>[4x]MARIIENNVGGVALTFDDVLLRPEFSNVLPRDIDISTRIAKDFTLNLPIMSAAMDQVTDSRLAIAMAQAGGLGVIHRNFSPSEQVAQVHQVKKFESGGVKDIERSQLNPNATKDSKGRLRVAAAVSVAKDIADRVGPLFDVNVDLVVVDTAHGHSQKVLDAVVQIKKNFPSLLVMAGNIATAEGALALIDAGADIIKVGIGPGSICTTRVVTGVGCPQLSAIMSVVEVAERAGVAIVADGGIRFSGDIAKAIAAGSACVMIGSLLAGTDESPGDIFLYQGRSFKSYRGMGSVAAMERGSSARYSQDGVTDVLKLVPEGIEGRVPYKGPIASVLHQMSGGLKSSMGYVGASNIEEFQKKANFIRVSVAGLRESHVHDVKITRESPNYSETI

Inosine 5′-monophosphate dehydrogenase (IMPDH) is the first and rate-limiting step in guanine nucleotide biosynthesis, controlling the gateway to guanine nucleotides. IMPDH catalyzes the oxidation of inosine 5′-monophosphate to xanthosine 5′-monophosphate (XMP) with a concomitant reduction of NAD+ to NADH. A monomer consists of two domains, namely, the catalytic domain, which is an eight-fold β/α barrel, and a subdomain, including two tandem cystathione-synthetase motifs (CBS domain or Bateman domain), which protrudes from the corners of the homotetramer. IMPDH is also a promising target for antibacterial drug discovery.

In this study, a CLas IMPDH variant without the CBS domain (CLas IMPDHΔ98-201) was designed. To get the CBS deletion construct, 104 residues (98-201aa) were replaced with a G amino acid, and the catalytic residue Cys309 was completely conserved. The crystal structure of CLas IMPDHΔ98-201 was determined in the apo form. Crystals of CLas IMPDHΔ98-201 appeared after 3 days at 293 K. The resolution of the diffracting crystal was 2.55 Å. Finally, the structure was refined to 2.55 Å resolution by using the PHENIX software. This crystal protein existed as a homotetramer, which is well conserved in other IMPDHs. The space group of CLas IMPDHΔ98-201 was C121, and the unit-cell parameters for CLas IMPDHΔ98-201 were a = 143.13, b = 134.86, and c = 85.62 Å. A comparison of the structures of CLas IMPDHΔ98-201 and BaIMPDHΔ95-200 showed that the structure of CLas IMPDHΔ98-201 was highly similar to that of BaIMPDHΔ95-200 in its apo form. The RMSD of CLas IMPDHΔ98-201 and BaIMPDHΔ95-200 was 0.929 Å. The flap loop and a C-terminal loop are not visible in the electron density. The steady-state kinetics parameters of CLas IMPDHΔ98-201 were similar to those of other IMPDHs, suggesting that deleting the CBS domain would not affect the CLas IMPDHΔ98-201 catalytic properties.>[2x]NRT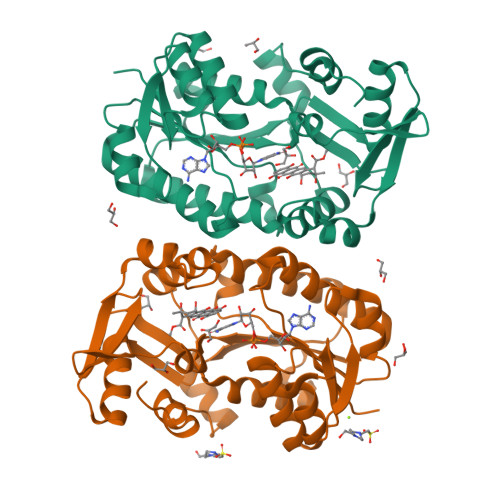ILVTGATGTQGGATVRALLARGRPVRALVRDPGTDAARALAAAGVSLVTGDLNDQASLRAAMADVHGVFSVQTFMTPGGLGAELRQGRAVADAAAATGVRHVVYSSVGGADRASGVPHFETKWTIERHLRSLGVPTTVLRPTFFMDNFAAWGPQAVDGTLVVRLPLKPQTRVQLIAAEDIGVFAATAFDDPDTYVGAALELAGDELTGPELAARFGELAGMPARFEERSLDEAAADPWIPYSHEIAVMFEWFQTDGYAADIAALRARHPGLRTFADWLRAIGWRVP> LTAQELNEDMPSKMLEPKNPQAPKNITVYDYYTRKFKTDELVDQMIVHFSMDGDYIWKESNEYKTQEEIRDTKKALIKEAMRKQESEEPGANHDEEAIKQTLRNKFNYNTRECQTINPSIRERGVSTEPPPSDTICGNITQWEIFDAYYAEIMKDHQIENKKKKEVDQDKKQDQSMYSTSFKR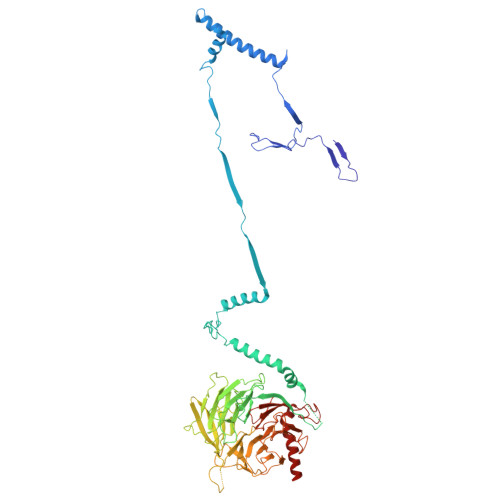CCKIMERMVVQNDQEDKYHDYRYYWSQGDNLEAGKNEGHLLPIWRFSNEKQRKKNVTSICWNPLYPDLFAVSLGSYDFTKQRMGLICLYSLKNTTHPEYAFNCEAGVMCLDFHPKSAALLAVGLYDGTVLVYDIRNKHKKPIYQSTVRNQKHTDPVWQVKWNPDTSKNYNFYSISSDGRVMNWILMKNKLEPEEVILLRLVGKNEEESTLIGLACGLCFDFNKFEPHIFLVGTEEGKIHKCSRAYSGQYQETYNGHLLAVYKVKWNNFHPRTFISASADWTVRIWDSKYTSQIICFDLSMMVVDAVWAPYSSTVFACATMDKVQVYDLNVDKLNKLAEQKIVKQPKLTNLSFNYKDPILLVGDSHGGVTLVKLSPNLCKSGPEIKQTEDKKAMEEFKNVKIEDYEREKMENL> MPVTINNFNYNDPIDNNNIIMMEPPFARGTGRYYKAFKITDRIWIIPERYTFGYKPEDFNKSSGIFNRDVCEYYDPDYLNTNDKKNIFLQTMIKLFNRIKSKPLGEKLLEMIINGIPYLGDRRVPLEEFNTNIASVTVNKLISNPGEVERKKGIFANLIIFGPGPVLNENETIDIGIQNHFASREGFGGIMQMKFCPEYVSVFNNVQENKGASIFNRRGYFSDPALILMHQLIYVLHGLYGIKVDDLPIVPNEKKFFMQSTDAIQAEELYTFGGQDPSIITPSTDKSIYDKVLQNFRGIVDRLNKVLVCISDPNININIYKNKFKDKYKFVEDSEGKYSIDVESFDKLYKSLMFGFTETNIAENYKIKTRASYFSDSLPPVKIKNLLDNEIYTIEEGFNISDKDMEKEYRGQNKAINKQAYEEISKEHLAVYKIQMCKSVKAPGICIDVDNEDLFFIADKNSFSDDLSKNERIEYNTQSNYIENDFPINELILDTDLISKIELPSENTESLTDFNVDVPVYEKQPAIKKIFTDENTIFQYLYSQTFPLDIRDISLTSSFDDALLFSNKVYSFFSMDYIKTANKVVEAGLFAGWVKQIVNDFVIEANKSNTMDKIADISLIVPYIGLALNVGNETAKGNFENAFEIAGASILLEFIPELLIPVVGAFLLESYIDNKNKIIKTIDNALTKRNEKWSDMYGLIVAQWLSTVNTQFYTIKEGMYKALNYQAQALEEIIKYRYNIYSEKEKSNINIDFNDINS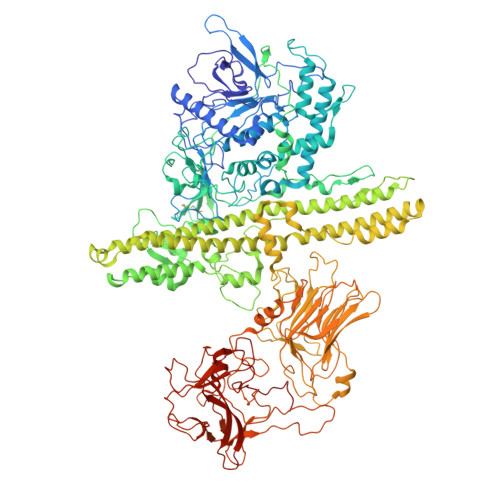KLNEGINQAIDNINNFINGCSVSYLMKKMIPLAVEKLLDFDNTLKKNLLNYIDENKLYLIGSAEYEKSKVNKYLKTIMPFDLSIYTNDTILIEMFNKYNSEILNNIILNLRYKDNNLIDLSGYGAKVEVYDGVELNDKNQFKLTSSANSKIRVTQNQNIIFNSVFLDFSVSFWIRIPKYKNDGIQNYIHNEYTIINCMKNNSGWKISIRGNRIIWTLIDINGKTKSVFFEYNIREDISEYINRWFFVTITNNLNNAKIYINGKLESNTDIKDIREVIANGEIIFKLDGDIDRTQFIWMKYFSIFNTELSQSNIEERYKIQSYSEYLKDFWGNPLMYNKEYYMFNAGNKNSYIKLKKDSPVGEILTRSKYNQNSKYINYRDLYIGEKFIIRRKSNSQSINDDIVRKEDYIYLDFFNLNQEWRVYTYKYFKKEEMKLFLAPIYDSDEFYNTIQIKEYDEQPTYSCQLLFKKDEESTDEIGLIGIHRFYESGIVFEEYKDYFCISKWYLKEVKRKPYNLKLGCNWQFIPKDEGWTELEVLFQGPLEHHHHHH> MDETGKEL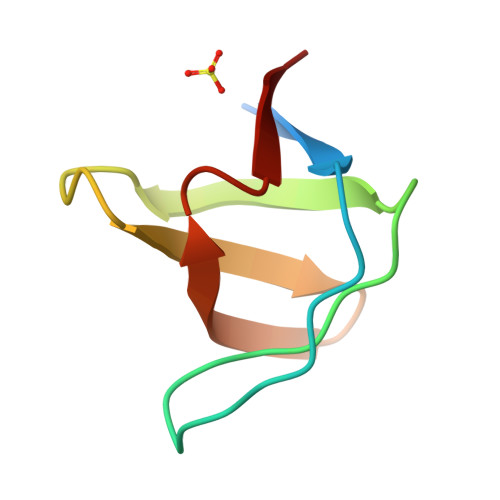VLALYDYQEKSPGEVTMKKGDILTLLNSTNKDWWKVEVNDRQGFVPAAYVKKLD> MYRDLVLNPQNRSVNRGDDEISLTKREYDLLNILMTNMNRVMTREELLSNV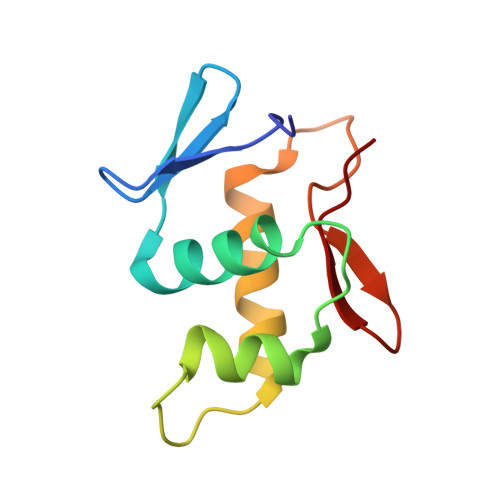WKYDEAVETNVVDVYIRYLRGKIDIPGKESYIQTVRGMGYVIREK>MTRTLPPGVSDERFD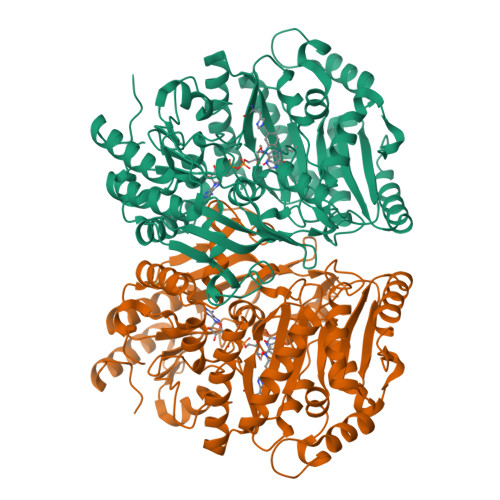AALQRFRDVVGDKWVLSTADELEAFRDPYPVGAAEANLPSAVVSPESTEQVQDIVRIANEYGIPLHPVSTGKNNGYGGAAPRLSGSVIVKTGERMNRILEVNEKYGYALLEPGVTYFDLYEYLQSHDSGLMLDCPELGWGSVVGNTLDRGVGYTPYGDHFMWQTGLEVVLPQGEVMRTGMGALPGSDAWQLFPYGFGPFPDGMFTQSNLGIVTKMGIALMQRPPASQSFLITFDKEEDLEQIVDIMLPLRINMAPLQNVPVLRNIFMDAAAVSKRTEWFDGDGPMPAEAIERMKKDLDLGFWNFYGTLYGPPPLIEMYYGMIKEAFGKIPGARFFTHEERDDRGGHVLQDRHKINNGIPSLDELQLLDWVPNGGHIGFVPVSAPDGREAMKQFEMVRNRANEYNKDYMASFIIGLREMYHVCLFIYDTADPEAREEILQMTKVLVREAAEAGYGEYRTHNALMDDVMATFNWGDGALLKFHEKIKDALDPNGIIAPGKSGIWPQRFRGQNL[8x]>[3x]MSLTQAQGAQQYVNINPPMPSDTPGKIEVLEFFAYTCPHCAAIEPMVEDWAKTAPQDV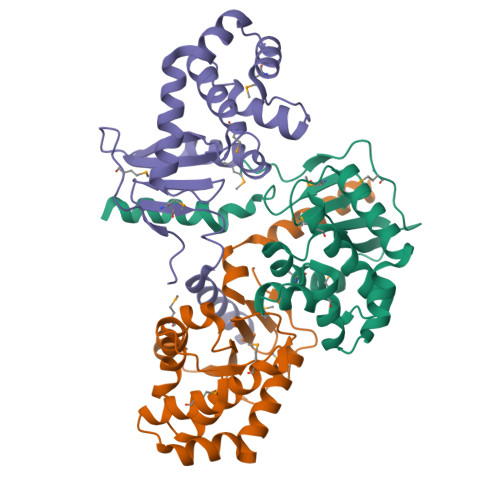VLKQVPIAFNAGMKPLQQLYYTLQALERPDLHPKVFTAIHTERKRLFDKKAMGEWAASQGVDRAKFDSVFDSFSVQTQVQRASQLAEAAHIDGTPAFAVGGRYMTSPVLAGNDYAGALKVVDQLIVQSREGHHHHHH>MSLSKPLFIFEMANNHMGNVEHGVALIRAIRESCQGFDFDFGFKLQYRNLDTFIHSSFKGRDDVKYVKRFEETRLQPEQMQKLVAEMKANGFKAICTPFDEESVDLIEAHGIEIIKIASCSFTDWPLLERIARSDKPVVASTAGARREDIDKVVSFMLHRGKDLTIMHCVAEYPTPDDHLHLARIKTLRQQYAGVRIGYSTHEDPDLMEPIMLAVAQGATVFEKHVGLPTDQYGINNYSANPEQVRRWLAAAARALAMLGDGEDDAVSETEQASLRSLRRGVFATRPVAAGEALTADNVSFAFPPVEGQL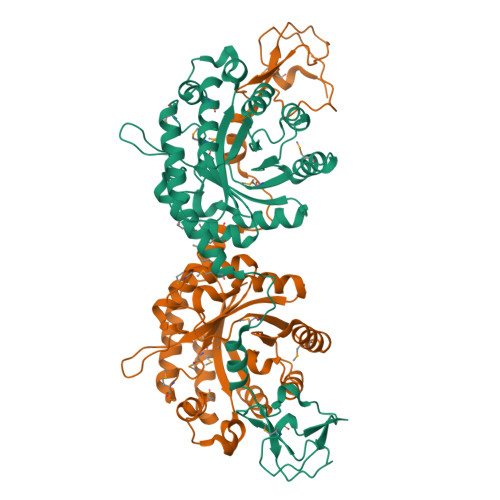TANEWSKYVRYTAKTPIAADAPVMAADLEPVNEGHHHHHH[2x]> MTKINLATLSVIGFLGSASIAQAECGEVSITEMNWASASVVTTVATFLMEQGYGCAVTVVPSSTVPAVTSVSETGEPDILTELWLSSLPNYAKLEAQGTVRTLTEVLSDGGQEGWWVPQYLAEAHPEVTTIEGILANPDLVGGRFHRSPDGWAAAIVDSSLAKAWDLEGNGIEVFAHGSGETLATSIAAAYADREPWFGYYWAPTSVLGKFPMVMVDLGEFDADIHACNSKADCANVGKSPYPRARVITAVTPGFAEENPEI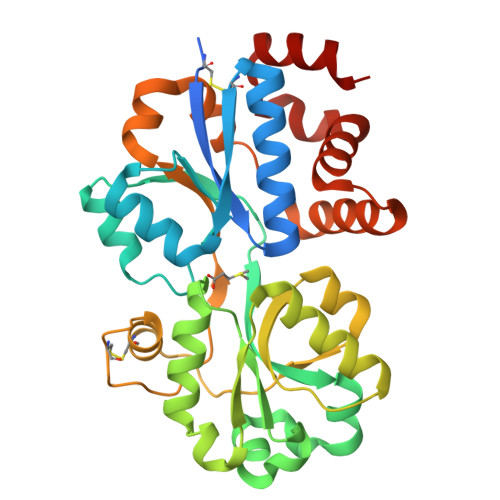IEMLSNLSFTNDQMGAILAWQEENGASSEEAAVWFLSNNSDIWAGWVNDAARENLAALIP>[2x]IRLPPEVNRILYIRNLPYKITAEEMYDIFGKYGPIRQIRVGNTPETRGTAYVVYEDIF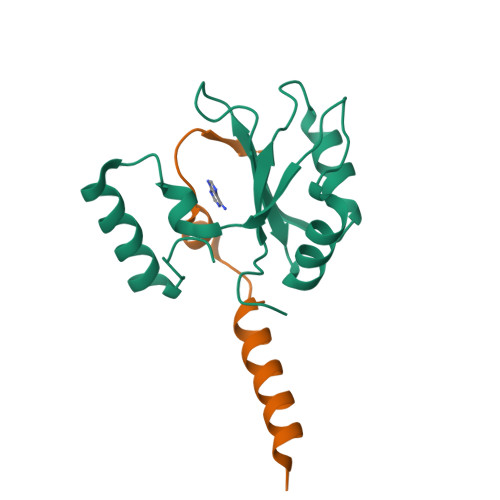DAKNAVDHLSGFNVSNRYLVVLYYNANRAFQKMDTKKKEEQLKLLKEKYGINTDPPK;>[2x]SMTPEQLQAWRWEREIDERNRPLSDEELDAMFPEGYKVL> MTDNKIKNEDGKLELIINAAQKRFAHYGLCKTTMNEIASDVGMGKASLYYYFPDKETLFEAVIKKEQNVFFDEMDKILNSGIDATALLKKYVKLRSLHFRHLLNLSKLRSDFFHNTKPVFAKAFESFKQKEVEIVAGIIQYGITTKEFKRGNKHENAEFLVHLLLGVRMVKLKYKEINDFDESDYEDLDKNMCKVA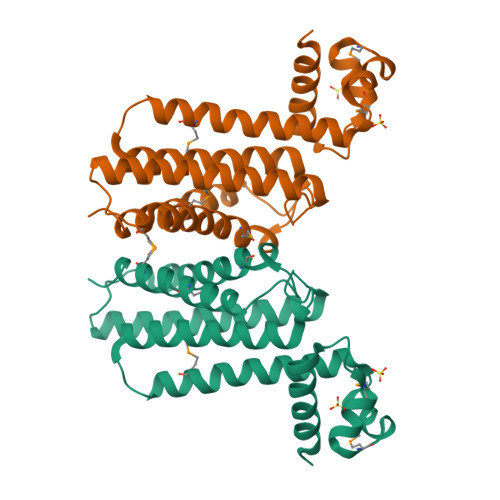GMFLKEIQTEVASRENLYFQ> MQNLFTKDVTVIEGEVATI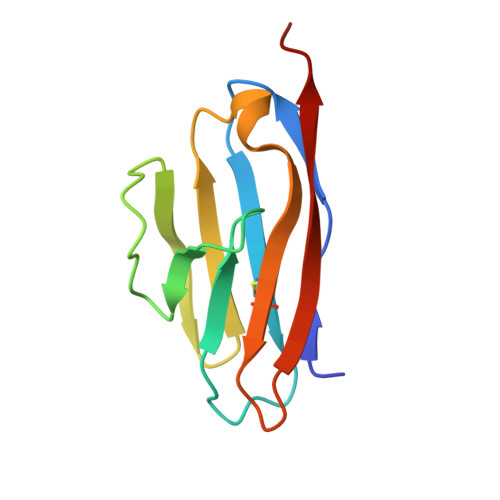SCQVNKSDDSVIQLLNPNRQTIYFRDFRPLKDSRFQLLNFSSSELKVSLTNVSISDEGRYFCQLYTDPPQESYTTITVLVPP>[3x]MKRDGHTHTEFCPHGTHDDVEEMVLKAIELDFDEYSIVEHAPLSSEFMKNTAGDKEAVTTASMAMSDLPYYFKKMNHIKKKYASDLLIHIGFEVDYLIGYEDFTRDFLNEYGPQTDDGVLSLHFLEGQGGFRSIDFSAEDY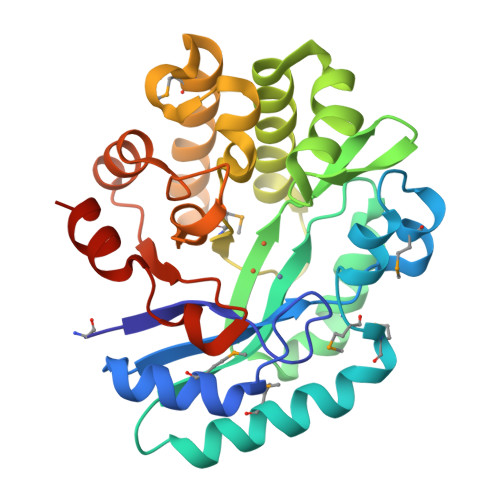NEGIVQFYGGFEQAQLAYLEGVKQSIEADLGLFKPRRMGHISLCQKFQQFFGEDTSDFSEEVMEKFRVILALVKKRDYELDFNTAGLFKPLCGETYPPKKIVTLASELQIPFVYGSDSHGVQDIGRGYSTYCQKLEHHHHHH>[2x]SRAPAPATPHAPDHSPAPNSPTLTRPPEGPKFPRVKNWELGSITYDTLCAQSQQDGPCTPRRCLGSLVLPRKLQTRPSPGPPPAEQLLSQARDFINQYYSSIKRS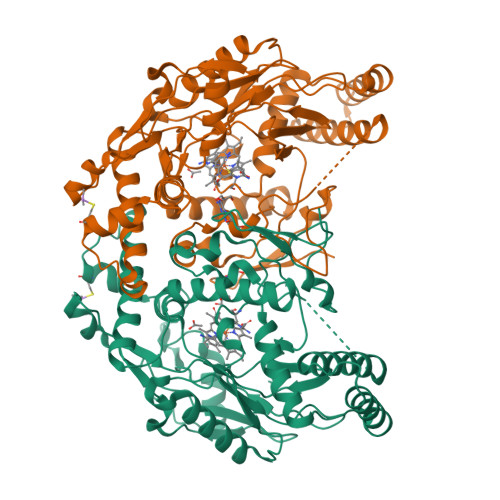GSQAHEERLQEVEAEVASTGTYHLRESELVFGAKQAWRNAPRCVGRIQWGKLQVFDARDCSSAQEMFTYICNHIKYATNRGNLRSAITVFPQRAPGRGDFRIWNSQLVRYAGYRQQDGSVRGDPANVEITELCIQHGWTPGNGRFDVLPLLLQAPDEAPELFVLPPELVLEVPLEHPTLEWFAALGLRWYALPAVSNMLLEIGGLEFSAAPFSGWYMSTEIGTRDLCDPHRYNILEDVAVCMDLDTRTTSSLWKDKAAVEINLAVLHSFQLAKVTIVDHHAATVSFMKHLDNEQKARGGCPADWAWIVPPISGSLTPVFHQEMVNYILSPAFRYQPDPW> KGSVVIVGRIVLSGKP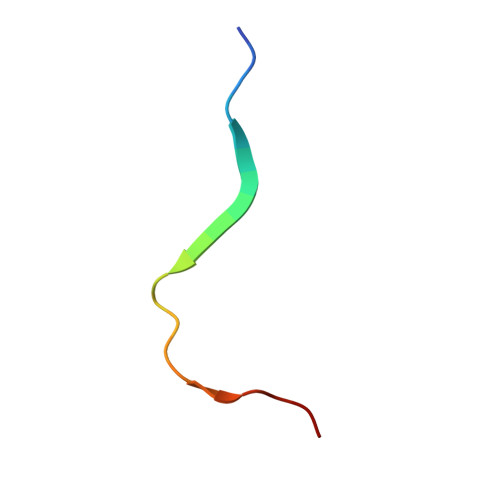AIIPKK> QLTIEVLVTVDGVNFRTVVLN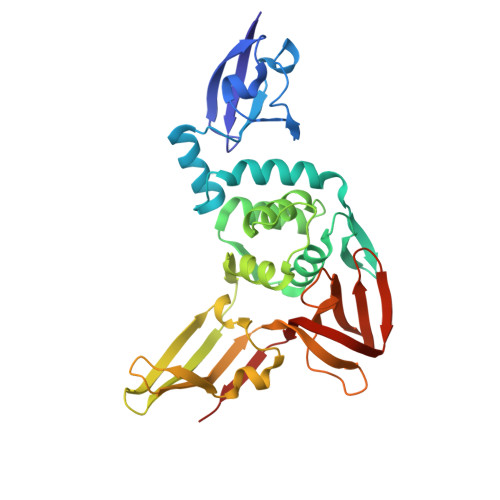NKNTYRSQLGCVFFNGADISDTIPDEKQNGHSLYLADNLTADETKALKELYGPVDPTFLHRFYSLKAAVHGWKMVVCDKVRSLKLSDNNCYLNAVIMTLDLLKDIKFVIPALQHAFMKHKGGDSTDFIALIMAYGNCTFGAPDDASRLLHTVLAKAELCCSARMVWREWCNVCGIKDVVLQGLKACCYVGVQTVEDLRARMTYVCQCGGERHRQLVEHTTPWLLLSGTPNEKLVTTSTAPDFVAFNVFQGIETAVGHYVHARLKGGLILKFDSGTVSKTSDWKCKVTDVLFPGQKYSSDCN> MRVPFSWLKAYVPELESPEVLEERLAGLGFETDRIERVFPIPRGVVFARVLEAHPIPGTRLKRLVLDAGRTVEVVSGAENARKGIGVALALPGTELPGLGQKVGERVIQGVRSFGMALSPRELGVGEYGGGLLEFPEDALPPGTPLSEAWPEEVVLDLEVTPNRPDALGLLGLARDLHALGYALVEPEAALKAEALPLPFALKVEDPEGAPHFTLGYAFGLRVAPSPLWMQRALFAAGMRPINNVVDVTNYVMLERAQPMHAFDLRFVGEGIAVRRAREGERLKTLDGVERTLHPEDLVIAGWRGEESFPLGLAGVMGGAESEVREDTEAIALEVACFDPVSIRKTARRHGLRTEASHRFERGVDPLGQVPAQRRALSLLQALAGARVAEALLEAGSPKPPEAIPFRPEYANRLLGTSYPEAEQIAILKRLGCRVEGEGPTYRVTPPSHRLDLRLEEDLVEEV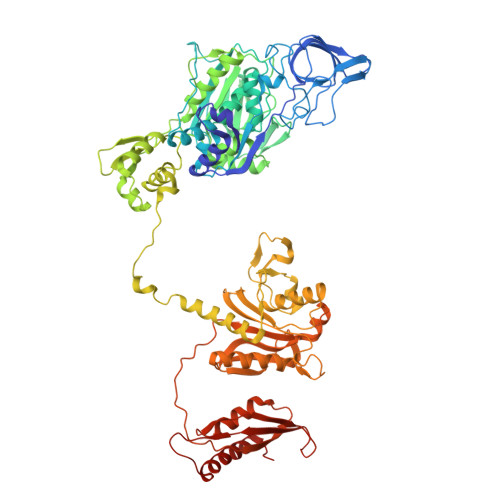ARIEGYETIPLALPAFFPAPDNRAVEAPYRKEQRLREVLSGLGFQEVYTYSFMDPEDARRFRLDPPRLLLLNPLAPEKAALRTHLFPGLVRVLKENLDLDRPERALLFEVGRVFREREETHLAGLLFGEGVGLPWAKERLSGYFLLKGYLEALFARLGLAFRVEAEAFPFLHPGVSGRVLVEGEEVGFLGALHPEIAQELELPPVHLFELRLPLPDKPLAFQDPSRHPAAFRDLAVVVPAPTPYGEVEALVREAAGPYLESLALFDLYQGPPLPEGHKSLAFHLRFRHPKRTLRDEEVEEAVSRVAEALRARGFGLRGLDTP>[4x]IDPFTMSDLPCPPTNAERLHEFHRAIGAATPERPTPPPPELLRLR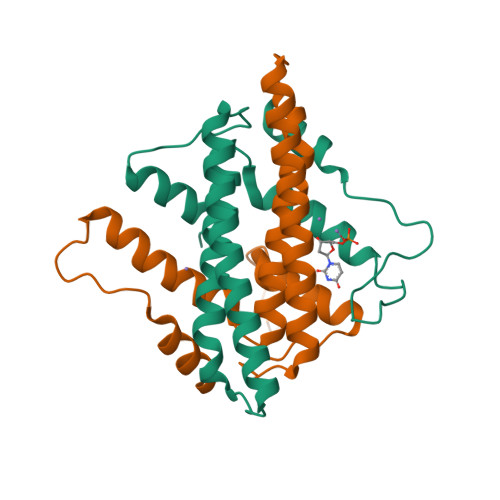QTLLDEASAEVRAEIDHLLARQAAGEALSAGDLAPLAHELADLLYVTYGALDQLGIDADAVFAEVHRANLSKASGPRRADGKQLKPEGWRPADVRGVIERLQHA A protein involved in resistance against different pathogen groups, which is only present in monocot plants, is referred to as monocot chimeric jacalin (MCJ). As its name suggests, it is a fusion of two proteins, a jacalin-related lectin (JRL) and a dirigent protein (DIR) at the N-terminus. Therefore, the development of disease resistant plants is mandatory. It was shown that the rice (Oryza sativa) protein OsJAC1 enhances resistance against different bacterial and fungal plant pathogens in rice, barley, and wheat. Here, we report crystal structures for both individual domains and the complex of galactobiose with the DIR domain, which revealed a new carbohydrate binding motif for DIR proteins.

The isolated DIR domain of OsJAC1 presents as a trimer in the asymmetric unit of both crystal forms, featuring C3-symmetry with the same mode of interaction among constituent chains. All OsJAC1 DIR protomers show the canonical eight-stranded antiparallel β-barrel fold known from structurally characterized homologs. The length of the traced chain differs significantly between the molecules of the DIR trimers, particularly in the N-terminal regions. These show signs of enhanced dynamics, exhibiting different degrees of disorder in the crystal structures. Consequently, the average pairwise Cα RMS distance between chains, amounting to 0.79 and 0.90 Å for DIR-cf1 and -cf2, respectively, reduces to 0.45 and 0.39 Å if residues preceding Leu26 or following Cys153 are omitted. In either model, chain B has the highest amino acid sequence coverage. Interestingly, residues Lys6–Thr10 were found hydrogen-bonded to Gln20–Thr24 of an adjacent chain (chain A in cf1) in the same trimer, adding an extra antiparallel strand to the neighboring β-barrel. Similar to the JRL domain dimer, the DIR domain trimer is categorized as a stable assembly by PISA; the solvent-accessible surface buried at the binary interfaces amounts to approximately 900 Å2 per subunit, increasing to above 1400 Å2 if the swapped β-strand is considered. The OsJAC1-DIR domain revealed an eight-stranded antiparallel β-barrel fold with a wide-open putative binding area, which is surrounded by five loops.

>[3x]GSHMLESKLQITPCGMLVQGNQINFTKLYLHHTPAGPEQNQSAVTSNDKKIGLGCIVVNNWSVYDGIGSDAKLVAYAKGLHVFAGAWHNSFSLVFEDERLKGSTLQVMGLIVEEGDWAIVGGTGQFAMATGVILKKMQEQKQYGNIIELTIHGFCPLLKGS> MDP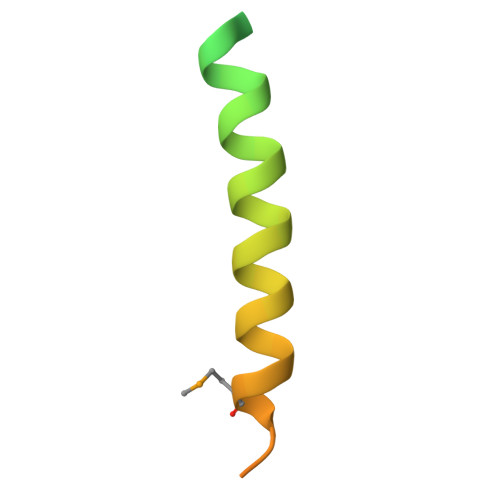PARKEKTKVKESVSRVEKAKQKSAQQELKQRQRAEIYALNRVMTELEQQQFDEFCKQMQPPGE>GSHMSKAFDLVVIGAGSGGLEAGWNAATLYGKRVAVVDVQTSHGPPFYAALGGTCVNVGCVPKKLMVTGAQYMDHLRESAGFGWEFDGSSVKANWKKLIAAKNEAVLDINKSYEGMFNDTEGLDFFLGWGSLESKNVVVVRETADPKSAVKERLQADHILLATGSWPQMPAIPGIEHCISSNEAFYLPEPPRRVLTVGGGFISVEFAGIFNAYKPPGGKVTLCYRNNLILRGFDETIREEVTKQLTANGIEIMTNENPAKVSLNTDGSKHVTFESGKTLDVDVVMMAIGRIPRTNDLQLGNVGVKLTPKGGVQVDEFSRTNVPNIYAIGDITDRLMLTPVAINEGAALVDTVFGNKPRKTDHTRVASAVFSIPPIGTCGLIEEVAAKEFEKVAVYMSSFTPLMHNISGSKYKKFVAKIVTNHSDGTVLGVHLLGDGAPEIIQAVGVCLRLNAKISDFYNTIGVHPTSAEELCSMRTPSYYYVKGEKMEKLPDSNL[2x]

Trypanothione reductase (TR) is a key factor in the redox homeostasis of trypanosomatid parasites, critical for survival in the hostile oxidative environment generated by the host to fight infection. In the case of the Trypanosomatidae, redox homeostasis relies on the dithiol trypanothione (TSH), a peculiar variant of glutathione (GSH) in which two GSH molecules are joined by the polyamine spermidine. TSH is kept in the reduced state by the action of the NADPH/FAD-dependent protein trypanothione reductase, homolog to the human glutathione reductase (GR). TR is considered an attractive target for the development of new trypanocidal agents as it is essential for parasite survival but has no close homolog in humans.

Site 14–15 is located in close proximity to the NADPH binding cavity. The analysis of the unbound TbTR structure made by FTmap predicts a hot spot located at this site, although it does not stand out as a remarkable druggable site. In fact, Phe198 is located over the FAD and, in the apo conformation, its side chain is perpendicular to the isoalloxazine ring. Upon NADPH binding, the nicotinamide moiety inserts between FAD and Phe198 forming an aromatic sandwich in which the phenyl ring lays parallel to the FAD. Therefore, for the NADPH to bind to TbTR, it is essential that Phe198 is able to switch from its perpendicular position to a parallel one with respect to the FAD.> MDADVERAEQDVRRDLFDDLSEHEDSEDALSDASAGDPKSRKSAHERRQAKIAEQIRKLEAELVAKRAWTLAGEATAADR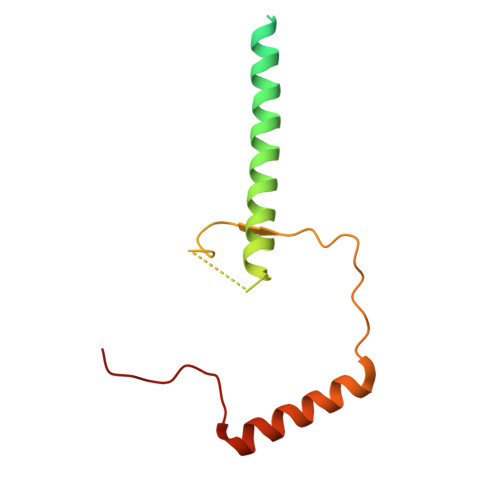PVNSLLGEDMEFDHVGKPVPVVTEEVSESIEELIKRRILAGEFDEVLRRRP> HHHHHHMNASPTPTATTTTEPATAVVRCRTRLARRVVAAVGPDGLLPAPCESRVLESALALALLTEERAEADATARLTAYLRTTLRTAPPDPFQCAVARAVLGGAGERGERVGDEGDMDAGTALDAGLDGFDHFTAGRKRLMFRTVLAALGATGFPAVPWEAYDTRPQQSWLHMEMKALKVLAAHGTGHPDVVRDEDWRALLPALEPGPAWECNNLAQLLALLALRHSPRHRPALGDVLKHVAGRLRPDGGMPYIDGMTVFTTAAAGLALSLLPAPPACVTPMADALALRRNPDGGYGFHSGVAQSDVEDTCYVLEFLRRAAPDRHRTAVAEAEGYLLALRNPDGGFPTFARGTSSEIAMTAAAASALAHDPDRREEVDEAVRYVVRHQRPDGTFERSWSRNATNAVFRAVLALTGVAAHGEERRSRARAAERALAHLAATQNGDGGWGHAEAEPSDPISTAYAVIALARGPRARPGGPLDRALAYLVERQHPDGGYRSRPDQAGPRPLLYD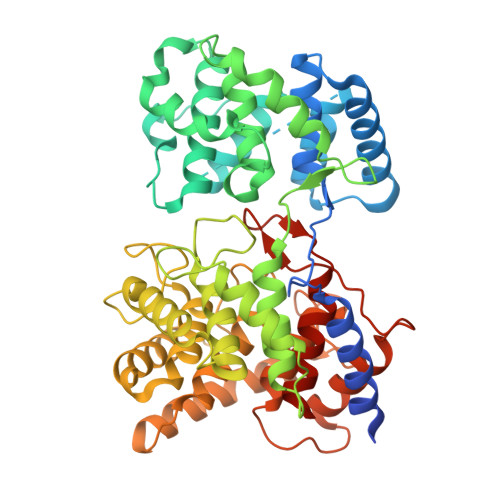VPALADVFVLLALAHATATPDPEGCSR> VFKKVLLTGTSEESFTAAADDAIDRAE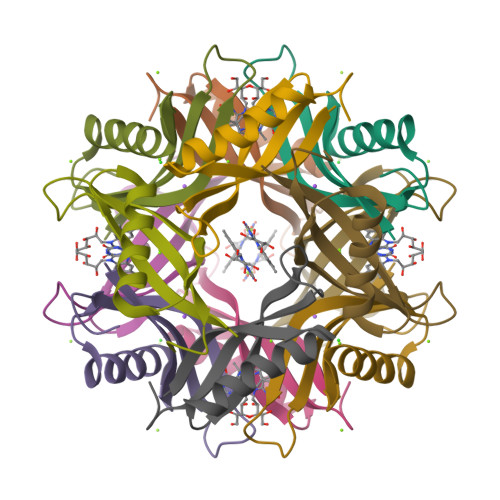DTLDNVVWAEVVDQGVEIGAVEERTYQTEVQVAFELDGSQ>GAMPHDPSFTPTQLAARAAYLLRGNDLGTMTTAAPLLYPHMWSWDAAFVAIGLAPLSVERAVVELDTLLSAQWRNGMIPHIVFANGVDGYFPGPARWATATLADNAPRNRLTSGITQPPVHAIAVQRILEHARTRGRSTRAVAEAFLDRRWGDLMRWHRWLAECRDRNERGRITLYHGWESGMDNSPRWDSAYANVVPGKLPEYQRADNVIITDPSQRPSDGEYDRYLWLLEEMKAVRYDDERLPSVMSFQVEDVFFSAIFSVACQ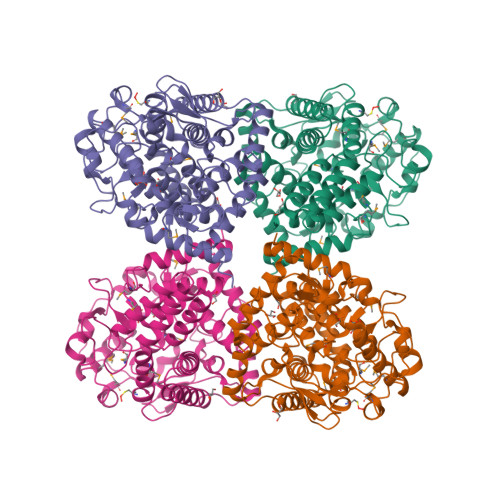VLAEIGEDYKRPHADVKDLYLWAERFRAGVVETTDQRTGAARDFDVLAEKWLVTETAAQFAPLLCGGLPHDRERALLKLLEGPRFCGHPDLKYGLIPSTSPVSRDFRPREYWRGPVWPVLTWLFSWCFARRGWAERARLLRQEGLRQASDGSFAEYYEPFTGEPLGSMQQSWTAAAVLDWLG[4x]4-1BB is not expressed on naive T cells but is rapidly upregulated after T-cell receptor engagement with cognate MHC:peptide complex expressed on antigen presenting cells. The 4-1BB binding partner, 4-1BBL, is a type II membrane protein of the TNF superfamily. The two leading molecules in the clinic are utomilumab (PF-05082566) and urelumab (BMS-663513). Consequently, we solved a series of structures that help us understand the structure–function relationship of the 4-1BB/4-1BBL signaling complex and how therapeutic antibodies could perturb this system.

To address this question directly we crystallized human 4-1BBL alone, determined the structure by molecular replacement, and refined to a resolution of 2.95 Å. SEC-MALS data showed that soluble 4-1BBL was trimeric in solution. Concordantly, the asymmetric unit contained three 4-1BBL molecules in trimeric assembly, with residues 89–244 visible in the electron density. Importantly, the 4-1BBL trimer again formed the canonical bell shape seen in every other TNFSF structure to date excepting the pinwheel 4-1BBL structure. Much like previously solved structures of TNFSF ligands, 4-1BBL adopts the jelly-roll fold typical of the TNF homology domain, with the inner and outer sheets of the beta sandwich consisting of anti-parallel beta strands A′AHCF and B′BGDE, respectively. While the structural jelly-roll fold of the protein core is well conserved between all three protomers, differences in conformation, discontinuous density and elevated B-factors can be seen in ligand loops A′B′ and DE suggesting a high degree of flexibility in the absence of a binding partner (inset). Analysis of binding interfaces with PISA shows that each protomer buries ∼1440 Å2. Comparison with our receptor-bound structure showed that the 4-1BBL trimer does in fact retain the overall bell-shaped arrangement in the absence of receptor. Specifically, the A′B′ loops in the ligand-only structure show varying degrees of disorder and variation between all three protomers. Hence, we believe our 4-1BBL structure represents the native unbound structure given its agreement with 4-1BB/4-1BBL complex as well as other structures of the TNFSF members either alone or in complex with their respective receptors.

>[3x]ARASPGSAASPRLREGPELSPDDPAGLLDLRQGMFAQLVAQNVLLIDGPLSWYSDPGLAGVSLTGGLSYKEDTKELVVAKAGVYYVFFQLELRRVVAGEGSGSVSLALHLQPLRSAAGAAALALTVDLPPASSEARNSAFGFQGRLLHLSAGQRLGVHLHTEARARHAWQLTQGATVLGLFRVTPEIPAGLPSPRSEGSHHHHHHHH>[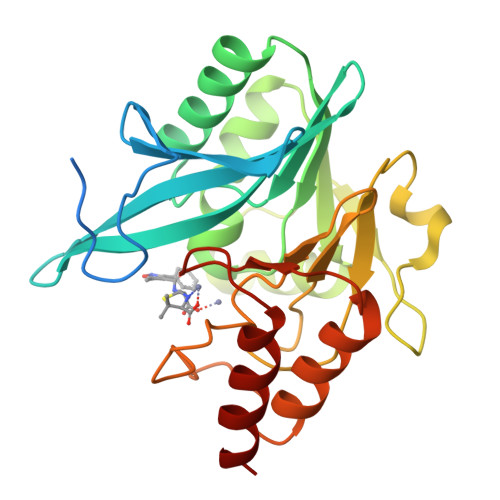2x]MELPNIMHPVAKLSTALAAALMLSGCMPGEIRPTIGQQMETGDQRFGDLVFRQLAPNVWQHTSYLDMPGFGAVASNGLIVRDGGRVLVVDTAWTDDQTAQILNWIKQEINLPVALAVVTHAHQDKMGGMDALHAAGIATYANALSNQLAPQEGMVAAQHSLTFAANGWVEPATAPNFGPLKVFYPGPGHTSDNITVGIDGTDIAFGGCLIKDSKAKSLGNLGDADTEHYAASARAFGAAFPKASMIVMSHSAPDSRAAITHTARMADKLR> GAGCGACCTGTACGGACATCA;> AACCTACCTGGCAGGACGACT;> CACGAGCCTGATCGGACAAGA;> TCTGATGTGGTAGG;> TGTCTTGTGGTCGC;> TTAGTCGTGGCT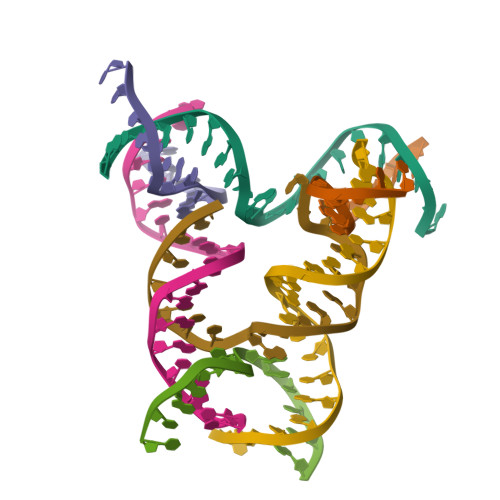CG;> ACACCGATCACCTGCCA> SMIPEVQKPLHEQL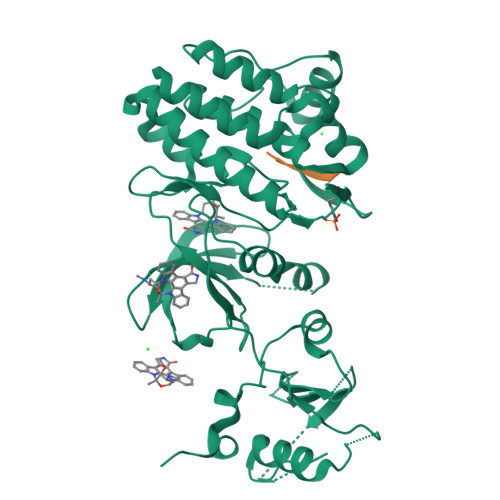WYHGAIPRAEVAELLVHSGDFLVRESQGKQEYVLSVLWDGLPRHFIIQSLDNLYRLEGEGFPSIPLLIDHLLSTQQPLTKKSGVVLHRAVPKDKWVLNHEDLVLGEQIGRGNFGEVFSGRLRADNTLVAVKSCRETLPPDLKAKFLQEARILKQYSHPNIVRLIGVCTQKQPIYIVMELVQGGDFLTFLRTEGARLRVKTLLQMVGDAAAGMEYLESKCCIHRDLAARNCLVTEKNVLKISDFGMSREEADGVYAASGGLRQVPVKWTAPEALNYGRYSSESDVWSFGILLWETFSLGASPYPNLSNQQTREFVEKGGRLPCPELCPDAVFRLMEQCWAYEPGQRPSFSTIYQELQSIRKRHR;> XIYESL~{S}-[4-(6-aminopurin-9-yl)butyl] ethanethioate | C11 H15 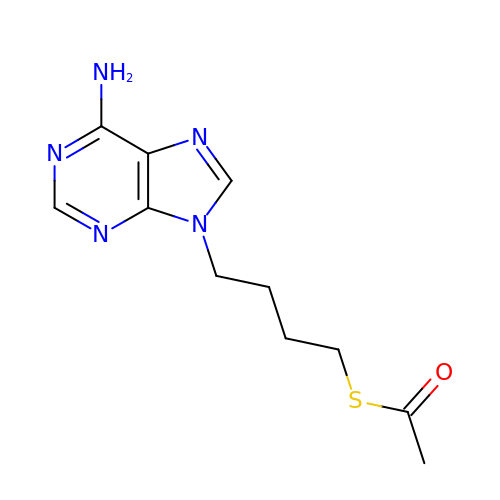N5 O S | MLUWWHOQAYWORL-UHFFFAOYSA-N> MSDDPIAASQAVVLSQAQAQNSQYALARTFATQKVSLEESVLSQVTTAIQTAQEKIVYAGNGTLSDDDRASLATDLQGIRDQLMNLANSTDGNGRYIFAGYKTEAAPFDQATGGYHGGEKSVTQQVDSARTMVIGHTGAQIFNSITSNAVPEPDGSDSEKNLFVMLDTAIAALKTPVEGNNVEKEKAAAAI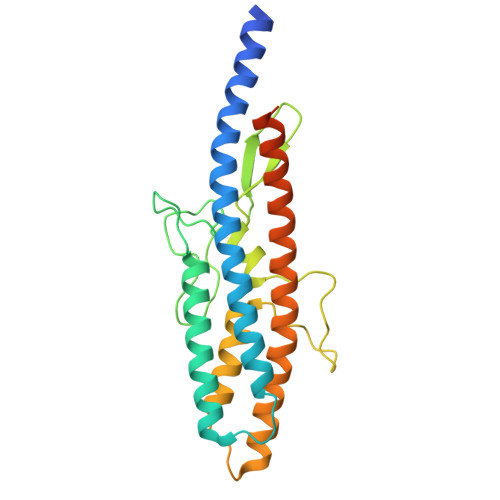DKTNRGLKNSLNNVLTVRAELGTQLSELSTLDSLGSDRALGQKLQMSNLVDVDWNSV>SMNPVQLDDFDAYIKDMAKDSDYKFSLQFEELKLIGLDIPHFAADLPLNRCKNRYTNILPYDFSRVRLVSMNEEEGADYINANYIPGYNSPQEYIATQGPLPETRNDFWKMVLQQKSQIIVMLTQCNEKRRVKCDHYWPFTEEPIAYGDITVEMISEEEQDDWACRHFRINYADEMQDVMHFNYTAWPDHGVPTANAAESILQFVHMVRQQATKSKGPMIIHCSAGVGRTGTFIALDRLLQHIRDHEFVDILGLVSEMRSYRMSMVQTEEQYIFIHQCVQLMWMKKKQQFCISDV[2x]

Protein tyrosine phosphatases (PTPs) play a critical role in regulating cellular functions by selectively dephosphorylating their substrates. The ∼280 residue PTP catalytic domain consists of an α/β structure, and biochemical and structural studies have led to a detailed understanding of the catalytic mechanism (Barford et al., 1994; Zhang, 2002). Key features of the domain include the PTP signature motif, the mobile Trp-Pro-Asp “WPD” loop that in the closed conformation positions the conserved and catalytically important aspartate residue, and the phosphotyrosine recognition loop. Here we report the crystal structures of 22 PTP domains, including two tandem-domain RPTP structures and a detailed structural comparison of this protein family.

Structural comparisons of all available PTP structures identified four main WPD loop conformations: a closed state, an intermediate state, an open state, and an atypically open state present in STEP, LYP, and GLEPP1. The atypically open state is associated in STEP with a stabilizing 310 helix C-terminal to the WPD loop (Eswaran et al., 2006) and in LYP and GLEPP1 an extra turn of helix α3 following the WPD loop. The presence of an atypically open state, catalytically nonactive conformation, in three PTPs from different subgroups suggests that this conformation may have significance for the family as a whole. Structural comparisons identified an atypically open WPD loop conformation in LYP, GLEPP1, and STEP (Eswaran et al., 2006), suggesting a regulatory role in diverse family members. This conformation represents an inactive conformation in which the WPD aspartate is moved far out of the active site. Low crystallographic temperature factors observed in this loop region suggest that the atypically open conformation is stable, and multiple crystal forms ruled out that the WPD loop assumed this conformation as a result of crystal contacts. In the first category are TCPTP, SHP1, SHP2, BDP1, LYP, PEST, PTPBAS, DEP1, MEG2, and GLEPP1, which have a “PTP1B-like” accessible pocket that harbors a basic residue corresponding to Arg24 of PTP1B. The new structural data and analysis presented here suggest that a secondary substrate-binding pocket, similar to that found in PTP1B, is present also in SHP2, BDP1, LYP, SHP1, TCPTP, MEG2, PTPBAS, DEP1, and GLEPP1. PTPs with particularly high enzymatic activity against generic substrates were RPTPσ and PTP subgroups R5, R3, NT1, NT2, NT3, NT4, and NT5. CD45 and members of subgroups R3 and R5 were extremely promiscuous and dephosphorylated most phosphopeptides with reasonable activity. Surprisingly, sedimentation velocity measurements showed that all single-domain RPTPs studied (IA2, IA2β, GLEPP1, DEP1, and STEP) were entirely monomeric in solution, as were tandem-domain receptor PTPs (RPTPα, CD45, RPTPɛ, and RPTPμ).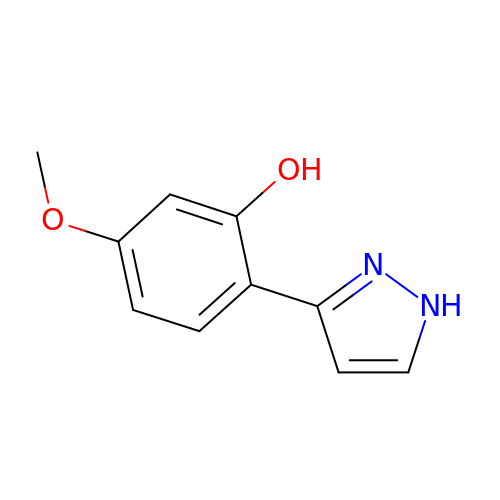5-methoxy-2-(1~{H}-pyrazol-3-yl)phenol | C10 H10 N2 O2 | KCSNRNYLTIFFOZ-UHFFFAOYSA-N> SADHRNGTQAANGKASAAGSAYSIDLNTFQTRLKAFYSHWDDRRTDLWGSSDAIAVACPPPSEDLRYLKSTALFLWLLGFEFPETIMVFTKKQIHVLCSQKKASILESVKKPAR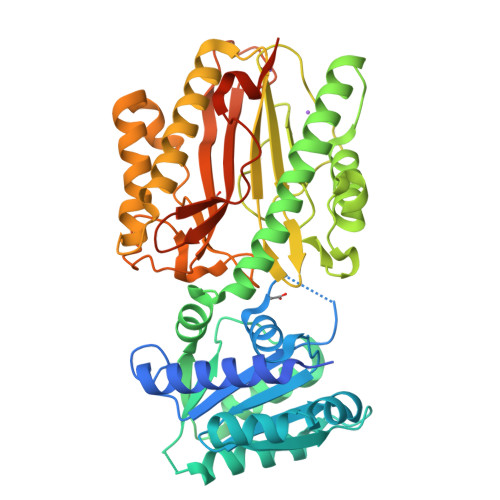ESVGVEIILHVKPKNDDGASSMDAIIRAIRAQSKSDGHDSSTVGHIAREEPEGRLLDLWAEKLKNSKFRLSDVANGFSALFAAKSNEEITYIKRAAYLTGSVMKNFVVTKLENVIDEEKKILHSTLMEETEKVILDPAKVNCKLKADNVDICYPPIFQSGGKFDLRPSAVSNDEALYYDSASVIICAVGARYKSYCSNIARTFLIDADPIQSKAYEVLLKAQEAVIGSLKPGNKLSAAYLAAVSVVEKDAPDMVSCLTKSAGTGIGIEFRESGLNINAKNDQIVKEGMVFNVSLGFQNLHCENSKSKNKVFSLLLADTIIINKDKTDVVTSIGSKALKDVAYSFNEDEEEEKPTSKAVPSGAEPLM>ELEVKNMDMKPGSTLKITGSIADGTDGFVINLGQGTDKLNLHFNPRFSESTIVCNSLDGSNWGQEQREDHLCFSPGSEVKFTVTFESDKFKVKL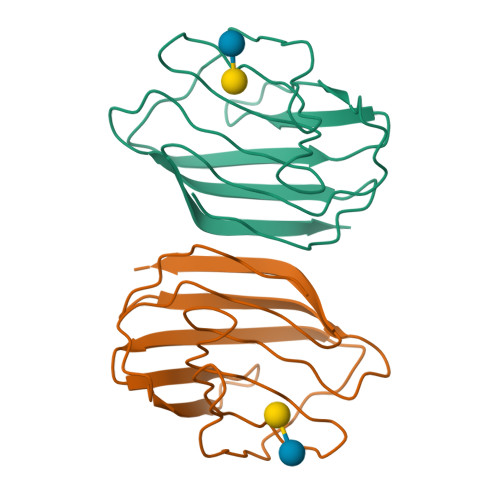PDGHELTFPNRLGHSHLSYLSVRGGFNMSSFKLKE[2x]> MFLNRLVKETSKAKRLFSMAQNNFARAGPYNPNRYKDYYIPRTLPKNEEIVEFVQSQHSVPASPIRNQRHINPVRESGPLPSYDGTYTMEDIRAVFYNTTVGRDYCYCQMDPEEIMRRVPGITRKEAEFITKLGLSPQEQVDFAYIAYNIGLDIFYFTNQMFVARQVVTNSKGEKVEVLWNAQCYEDIAQLNVGFAPVLESVDYHWEIF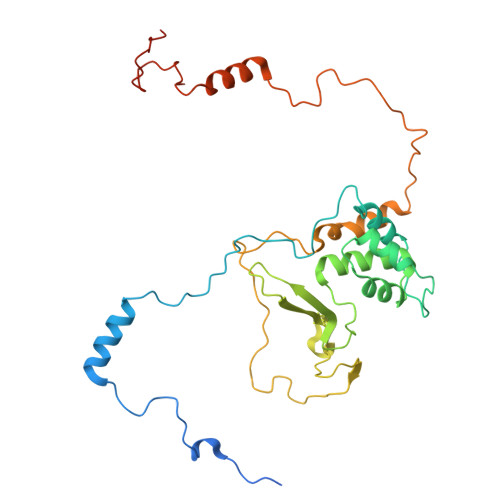LWADPPIKPNNDFDLNVPCTWFEYEQEWWMESCIQEDQFNLPEDERPYNTPRNPHCRKELWRSQDALQEEELMVNENWYPKNTQYNIYNQPDFIKPKSGSGAAADDIRI>[4x]MVSFKRYELPPLPYNYNALEPYIIEEIMKLHHQKHHNTYVKGANAALEKIE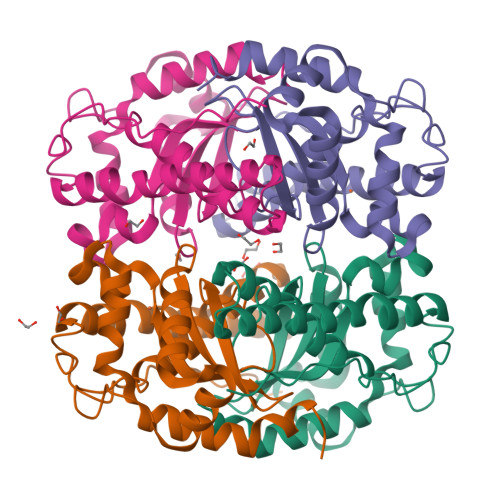KHLKGEIQIDVRAVMRDFSFNYAGHIMHTIFWPNMAPPGKGGGTPGGRVADLIEKQFGGFEKFKALFSAAAKTVEGVGWGVLAFDPLTEELRILQVEKHNVLMTAGLVPILVIDVWEHAYYLQYKNDRGSYVENWWNVVNWDDVEKRLEQALNNAKPLYLLPQ> MIKSALLVLEDGTQFHGRAIGATGSAVGEVVFNTSMTGYQEILTDPSYSRQIVTLTYPHIGNVGTNDADEESSQVHAQGLVIRDLPLIASNFRNTEDLSSYLKRHNIVAIADIDTRKLTRLLREKGAQNGCIIAGDNPDAALALEKARAFPGLNGMDLAKEVTTAEAYSWTQGSWTLTGGLPEAKKEDELPFHVVAYDFGAKRNILRMLVDRGCRLTIVPAQTSAEDVLKMNPDGIFLSNGPGDPAPCDYAITAIQKFLETDIPVFGICLGHQLLALASGAKTVKMKFGHHGGNHPVKDVEKNVVMITAQNHGFAVDEATLPANLRVTHKSLFDGTLQGIHRTDKPAFSFQGHPEASPGPHDAA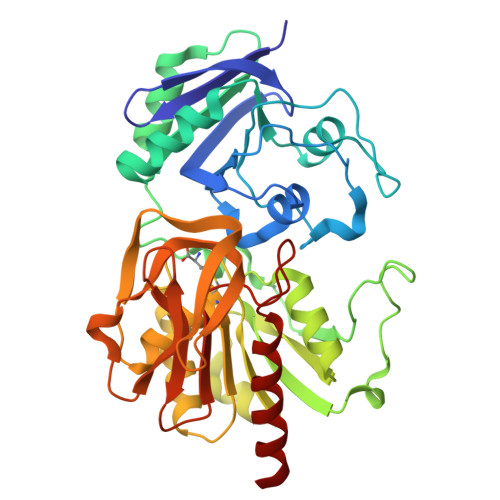PLFDHFIELIEQYRKTAK>MKSLSFMRVLEAVRTMLQEKGGLDVSIVMRNQVEMPTTMIEMIDQEEEESQTAWKEKYRFAIHHYTNEQDLAGVEKIDTLIQMGFILPEGYKLVAVRHCGKQNLVKENTLIHAKTSFEVSICRELKVKI[6x];>MAFEENLYCDYTPGAAKAVAGKDVILAVFNAAGDKLLAVAGQQGLTVNRSKDSIEITSKDTVGGWKSKIGGMKEWSIENDGLYVADAESHKELAKYFESDSPVCVKIINQASKKGLFGGLAIVADYSFEAPFDEAMTYSVKLDGMGALVDLTITEGGDQ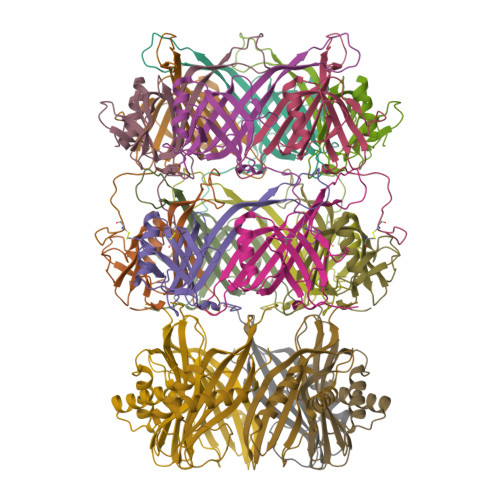MPGETPVAPAE[12x]>[12x]MRGSHHHHHHGSACMKRQGASSERKRARIPSGKAGAANGFLMEVCVDSVESAVNAERGGADRIELCSGLSEGGTTPSMGVLQ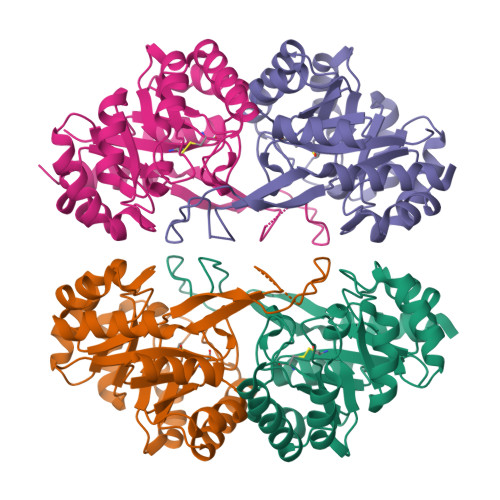VVKQSVQIPVFVMIRPRGGDFLYSDREIEVMKADIRLAKLYGADGLVFGALTEDGHIDKELCMSLMAICRPLPVTFHRAFDMVHDPMAALETLLTLGFERVLTSGCDSSALEGLPLIKRLIEQAKGRIVVMPGGGITDRNLQRILEGSGATEFHCSARSTRDSGMKFRNSSVAMGASLSCSEYSLKVTDVTKVRTLNAIAKNILV>MQQGQMAYSRAITVFSPDGRLFQVEYAREAVKKGSTALGMKFANGVLLISDKKVRSRLIEQNSIEKIQLIDDYVAAVTSGLVADARVLVDFARISAQQEKVTYGSLVNIENLVKRVADQMQQYTQYGGVRPYGVSLIFAGIDQIGPRLFDCDPAGTINEYKATAIGSGKDAVVSFLEREYKENLPEKEAVTLGI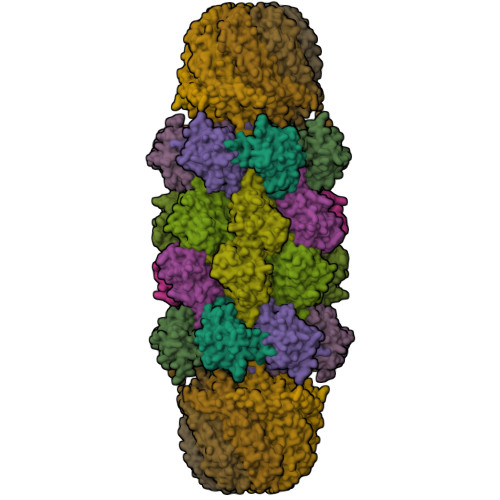KALKSSLEEGEELKAPEIASITVGNKYRIYDQEEVKKFL[7x];>MNQTLETGTTTVGITLKDAVIMATERRVTMENFIMHKNGKKLFQIDTYTGMTIAGLVGDAQVLVRYMKAELELYRLQRRVNMPIEAVATLLSNMLNQVKYMPYMVQLLVGGIDTAPHVFSIDAAGGSVEDIYASTGSGSPFVYGVLESQYSEKMTVDEGVDLVIRAISAAKQRDSASGGMIDVAVITRKDGYVQLPTDQIESRIRKLGLILHHHHHH[7x];>[7x]MHHHHHHPPKRAALIQNLRDSYTETSSFAVIEEWAAGTLQEIEGIAKAAAEAHGVIRNSTYGRAQAEKSPEQLLGVLQRYQDLCHNVYCQAETIRTVIAIRIPEHKEEDNLGVAVQHAVLKIIDELEIKTLGSGEKSGSGGAPTPIGMYALREYLSARSTVEDKLLGSVDAESGKTKGGSQSPSLLLELRQIDADFMLKVELATTHLSTMVRAVINAYLLNWKKLIQPRTGSDHMVS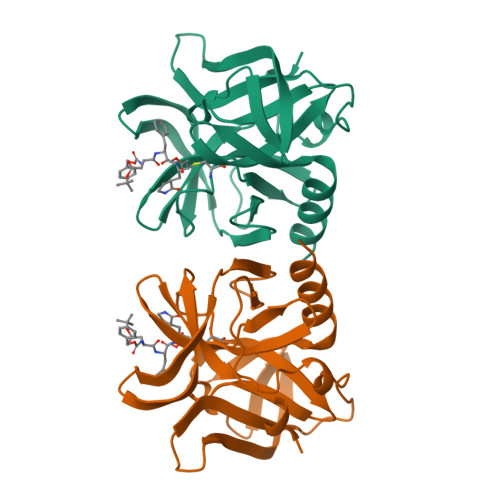> GPAFEFAVAMMKRNSSTVKTEYGEFTMLGIYDRWAVLPRHAKPGPTILMNDQEVGVLDAKELVDKDGANLELTLLKLNRNEKFRDIRGFLAKEEVEVNEAVLAINTSKFPNMYIPVGQVTEYGFLYLGGTPTKRMLMYNFPTRAGQCGGVLMSTGKVLGIHVGGNGHQGFSAALLKHYFNDEQ> GDRVKKLINSQISLLIGKGLHEFDSLRDPEVNDFRTKMRQFCEEAAAHRQQLGWVEWLQYSFPLQLEPSARGWRAGLLRVSNRALLVNVK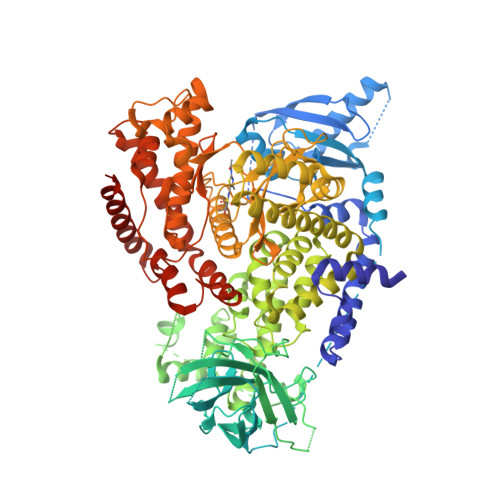FEGSEESFTFQVSTKDMPLALMACALRKKATVFRQPLVEQPEEYALQVNGRHEYLYGNYPLCHFQYICSCLHSGLTPHLTMVHSSSILAMRDEQSNPAPQVQKPRAKPPPIPAKKPSSVSLWSLEQPFSIELIEGRKVNADERMKLVVQAGLFHGNEMLCKTVSSSEVNVCSEPVWKQRLEFDISVCDLPRMARLCFALYAVVEKAKKARSTKKKSKKADCPIAWANLMLFDYKDQLKTGERCLYMWPSVPDEKGELLNPAGTVRGNPNTESAAALVIYLPEVAPHPVYFPALEKILELGRHGERGRITEEELQLREILERRGSGELYEHEKDLVWKMRHEVQEHFPEALARLLLVTKWNKHEDVAQMLYLLCSWPELPVLSALELLDFSFPDCYVGSFAIKSLRKLTDDELFQYLLQLVQVLKYESYLDCELTKFLLGRALANRKIGHFLFWHLRSEMHVPSVALRFGLIMEAYCRGSTHHMKVLMKQGEALSKLKALNDFVKVSSQKTTKPQTKEMMHMCMRQETYMEALSHLQSPLDPSTLLEEVCVEQCTFMDSKMKPLWIMYSSEEAGSAGNVGIIFKNGDDLRQDMLTLQMIQLMDVLWKQEGLDLRMTPYGCLPTGDRTGLIEVVLHSDTIANIQLNKSNMAATAAFNKDALLNWLKSKNPGEALDRAIEEFTLSCAGYCVATYVLGIGDRHSDNIMIRESGQLFHIDFGHFLGNFKTKFGINRERVPFILTYDFVHVIQQGKTNNSEKFERFRGYCERAYTILRRHGLLFLHLFALMRAAGLPELSCSKDIQYLKDSLALGKTEEEALKHFRVKFNEALRESWKTKVNWLAHNVSKDNRQ>[2x]MDYKESCPSVSIPSSDEHREKKKRFTVYKVLVSVGRSEWFVFRRYAEFDKLY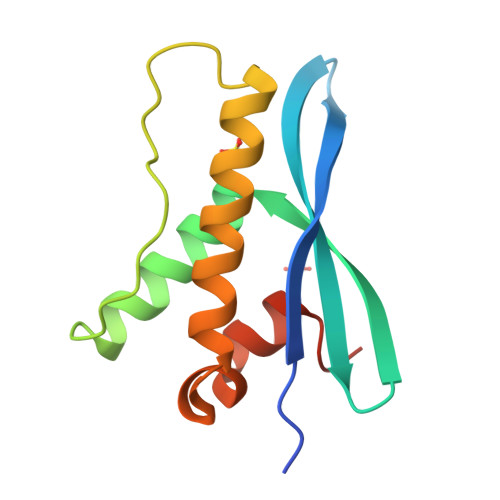NSLKKQFPAMALKIPAKRIFGDNFDPDFIKQRRAGLNEFIQNLVRYPELYNHPDVRAFLQMDSPRHQS> MASDYKDDDDKGALEVLFQGPSSPMAGNLVSWACKLCRSPEGFGPISFYGDFTQCFIDGVILNLSAIFMITFGIRDLVNLCKKKHSGIKYRRNWIIVSRMALVLLEIAFVSLASLNISKEEAENFTIVSQYASTMLSLFVALALHWIEYDRSVVANTVLLFYWLFETFGNFAKLINILIRHTYEGIWYSGQTGFILTLFQVITCASILLLEALPKKPLMPHQHIHQTLTRRKPNPYDSANIFSRITFSWMSGLMKTGYEKYLVEADLYKLPRNFSSEELSQKLEKNWENELKQKSNPSLSWAICRTFGSKMLLAAFFKAIHDVLAFTQPQLLRILIKFVTDYNSERQDDHSSLQGFENNHPQKLPIVRGFLIAFAMFLVGFTQTSVLHQYFLNVFNTGMYIKSALTALIYQKSLVLSNEASGLSSTGDIVNLMSVDVQKLQDLTQWLNLIWSGPFQIIICLYSLYKLLGNSMWVGVIILVIMMPLNSFLMRIQKKLQKSQMKYKDERTRVISEILNNIKSLKLYAWEKPYREKLEEVRNNKELKNLTKLGCYMAVTSFQFNIVPFLVSCCTFAVFVYTEDRALTTDLVFPALTLFNLLSFPLMIIPMVLNSFIEASVSIGRLFTFFTNEELQPDSVQRLPKVKNIGDVAINIGDDATFLWQRKPEYKVALKNINFQAKKGNLTCIVGKVGSGKTALLSCMLGDLFRVKGFATVHGSVAYVSQVPWIMNGTVKENILFGHRYDAEFYEKTIKACALTIDLAILMDGDKTLVGEKGISLSGGQKARLSLARAVYARADTYLLDDPLAAVDEHVARHLIEHVLGPNGLLHTKTKVLATNKVSALSIADSIALLDNGEITQQGTYDEITKDADSPLWKLLNNYGKKNNGKSNEFGDSSESSVRESSIPVEGELEQLQKLNDLDFGNSDAISLRRASDATLGSIDFGDDENIAKREHREQGKVKWNIYLEYAKACNPKSVCVFILFIVISMFLSVMGNVWLKHWSEVNSRYGSNPNAARYLAIYFALGIGSALATLIQTIVLWVFCTIHASKYLHNLMTNSVLRAPMTFFETTPIGRILNRFSNDIYKVDALLGRTFSQFFVNAVKVTFTITVICATTWQFIFIIIPLSVFYIYYQQYYLRTSRELRRLDSITRSPIYSHFQETLGGLATVRGYSQQKRFSHINQCRIDNNMSAFYPSINANRWLAYRLELIGSIIILGAATLSVFRLKQGTLTAGMVGLSLSYALQITQTLNWIVRMTVEVETNIVSVERIKEYADLKSEAPLIVEGHRPPKEWPSQGDIKFNNYSTRYRPELDLVLKHINIHIKPNEKVGIVGRTGAGKSSLTLALFRMIEASEGNIVIDNIAINEIGLYDLRHKLSIIPQDSQVFEGTVRENIDPINQYTDEAIWRALELSHLKEHVLSMSNDGLDAQLTEGGGNLSVGQRQLLCLARAMLVPSKILVLDQATAAVDVETDKVVQETIRTAFKDRTILTIAHRLNTIMDSDRIIVLDNGKVAEFDSPGQLLSDNKSLFYSLCMEAGLVNENGLVPRGSSAHHHHHHHHH

ATP-binding cassette (ABC) transporters catalyze the translocation of a wide range of substrates across membranes and support a variety of physiological processes including ion homeostasis, adaptative immune responses, lipid distribution, and detoxification. They consist of two cytosolic nucleotide-binding domains (NBDs) that can bind and hydrolyze ATP which promotes conformational changes in their transmembrane domains (TMDs). The ABCC family also expands the canonical ABC architecture with the addition of a long disordered link between NBD1 and TMD2 called the regulatory domain (R-domain) in some ABCC transporters. Some of the relevant transporters included in this family are CFTR, involved in chloride ion homeostasis; multidrug resistance protein 1 (MRP1) involved in the secretion of leukotrienes and drugs; the sulfonylurea receptor 1 (SUR1) a potassium channel that regulates insulin secretion; and the yeast cadmium factor 1, which is responsible for heavy metal and drug detoxification in yeast.

We expressed and purified the NBD2 Walker B mutant E1435Q Ycf1 in the Saccharomyces cerevisiae DSY5 strain and in the Materials and Methods section. After phosphorylation treatment with cAMP-PKA and size exclusion chromatography, cryo-EM grids were prepared as described in the Materials and Methods section. This approach yielded homogenous particles from which we identified a single inward-facing conformation in a 3.23 Å map. The overall conformation has previously been unobserved with a 40.0 Å separation between NBDs, ∼5 Å wider separation than the previous widest model (G668 on NBD1 and S1411 on NBD2). The high-quality map allowed the first-time modeling of four phosphorylation sites (S903, S908, T911, and S914) in a single ABC transporter R-domain. The S903 residue and its phosphate group make extensive interactions in a highly basic pocket defined by the surface of NBD1 (L619, K655, H803, K805, and K807) and R-insertion (615–643), especially at the K617 site, the latest being consistent with the R-insertion of CFTR in a proposed alternate conformation. Direct contacts amenable to ionic interaction are observed among three of the six residues in this cluster: the positively charged residues K617, K655, and K805 at 3.3, 3.4, and 2.5 Å respective distances to the phosphate oxygen group. The individual PKC, PKA, and CKII recognition motifs are shared by at least one residue to the next kinase motif in the R-domain sequence: R905 shared by PKC and PKA motif; S908 shared by PKA and CKII and T911 shared between two CKII motifs. This stabilized tetra-phosphorylated motif (PKC-PKA-CKII-CKII) makes a linear segment completely involved or bound to basic charges. The cryo-EM maps of the enriched tetra-phosphorylated Ycf1 also reveal a continuous R-domain density that encloses entirely around NBD1 in a path resembling previously published Ycf1 structures.>MSRRPTLRLGLDRDVYNIVLNLEQQGTDENGKRPRLTVDYVYDTIKRSNSSLARQKKRMLEDSIERVLAVRKEQAKAEEETDSDDLIEAQERERERQKAAQAQRDANLLNRQIAKSWGFASSPGAKAADGEKGTDTGSIATPAPATPAVAENMAADTPTTSTGPVLPASSTDRQPNGEPRPKKRKAAPKEIDRTPPTKVSILDIAGVDDTLQRLLKEVWFPLRGGEACEKMGYRYDNGVLLHGPSGCGKTTLAHAIAGSIGVAFIPVSAPSVIGGTSGESEKNIRDVFDEAIRLAPCLIFLDQIDAIAGRRESANKGMESRIVAEIMNGMDRIRQNTPLGKNVVVLAATNRPEFLDPAIRRRFSVEIDMGMPSERAREQILRSLTRDLSLADDINFKELAKMTPGYVGSDLQYVVKAAVSESFQANIDSLLAQARAKHPADHLANVSQPQRDWLLLEAHRDEEVSWPSTKITMEQFRKAVSLVQPASKREGFSTIPDTTWSHVGALEDVRKKLEMSIIGPIKNPELFTRVGIKPAAGILLWGPPGCGKTLVAKAVANESKANFISIKGPELLNKYVGESERAVRQLFSRAKSSAPCILFFDQMDALVPRRDDSLSDASARVVNTLLTELDGVGDRSGIYVIGATNRPDMIDEAIRRPGRLGTSIYVGLPSAEDRVKILKTLYRNTVKAPK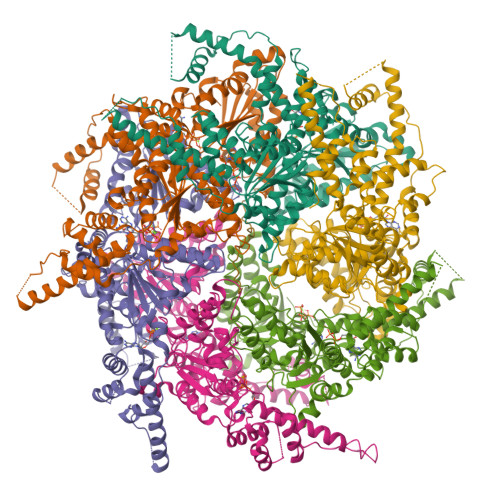KREGTNGEDVDMTDAAAEQQHQGTTDADLEKVALDLRCTGFSGADLGNLMQAAAQACLERVYTQRQQKRKEGGSVAEEEEIEPVITMEDWEKALNEVKPSVKDPEKYMHSGFAAALEHHHHHH[6x];> VVVVVVVVVVVVVVVVVVVVVVV>[2x]GHMSTPRQILAAIFDMDGLLIDSEPLWDRAELDVMASLGVDISRRNELPDTLGLRID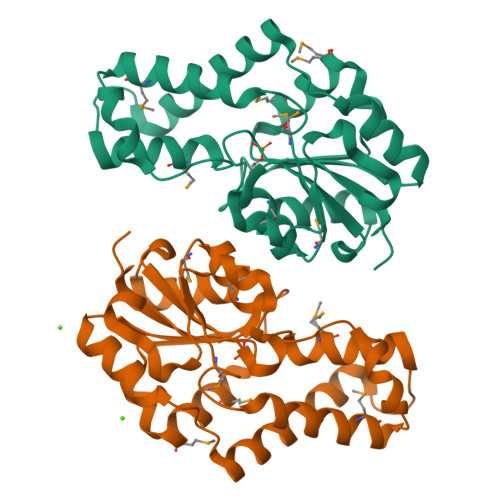MVVDLWYARQPWNGPSRQEVVERVIARAISLVEETRPLLPGVREAVALCKEQGLLVGLASASPLHMLEKVLTMFDLRDSFDALASAEKLPYSKPHPQVYLDCAAKLGVDPLTCVALEDSVNGMIASKAARMRSIVVPAPEAQNDPRFVLANVKLSSLTELTAKDLLGGS>MSTTNHDHHIYVLMGVSGSGKSAVASEVAHQLHAAFLDGDFLHPRRNIEKMASGEPLNDDDRKPWLQALNDAAFAMQRTNKVSLIVCSALKKHYRDLLREGNPNLSFIYLKGDFDVIESRLKARKGHFFKTQMLVTQF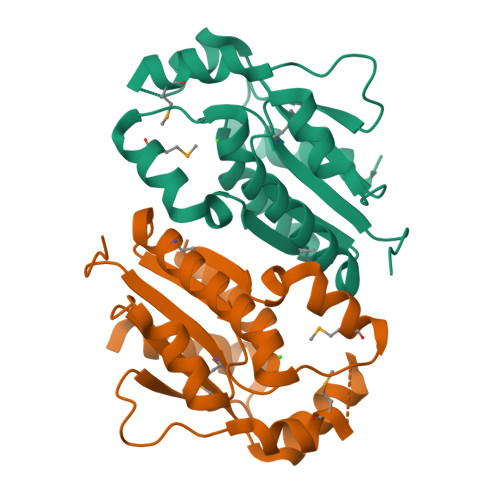ETLQEPGADETDVLVVDIDQPLEGVVASTIEVIKKGK[2x]>MNIYRYEENPLITPLDVKPIHEGFEVIGAFNGGVAEYNGEVLLLLRVAEKPVSEDPEIVLAPVYNAKNKELELQSFRLDDENYDFEDPRMIRSKAKLEGFSYLTSLSYIRIARSKDGHHFTLDEKPFLYPFNEYQTFGIEDARVTQIGDTYHVNFSAVSEFGVADALVTTKDFENLEYQGNIFAPENKDVLIFPEKINGKYYALHRPSLKSIGNLDIWIASSPDLRSFGDHRHLLGIRPGEYDSGRVGGGCVPIKTEEGWLILYHGATEENRYVMGAALLDLNDPTIVLKRTKTPILEPVADYEKNGFFGDVVFACGAIQEGDTLH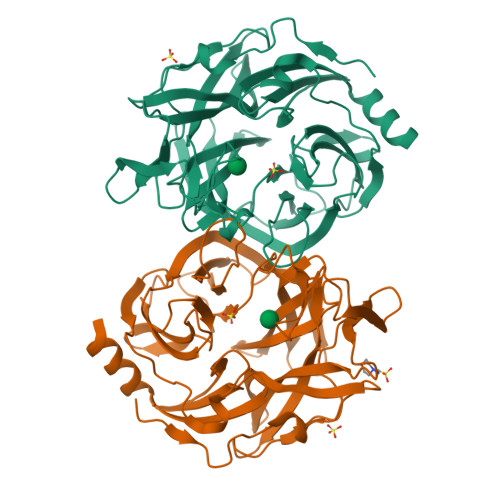MYYGVADTSMAGCDMKISEILHQLEVEAKLEHHHHHH[2x]> GSHMMFLVVGQGNPGERYARTRHNLGFMVLDRLGLSFRPRGEALVAEAEGGLFLKPLTYYNLTGRAVAPLARFYKIPPERILVVHDEMDLPLGRIRFKAGGSAAGNRGVLSIEEALGTRAFHR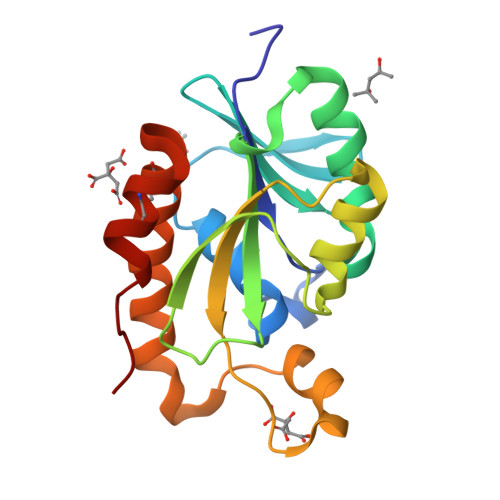LRLGIGKPPDPSRGAEYVLSPFREEELPVVERVLEAAKEAVWCWVREGLPPCAGRFNGLDLSLG>CGIFAYLNYHVPRTRREILETLIKGLQRLEYRGYDSAGVGFDGGNDKDWEANACKIQLIKKKGKVKALDEEVHKQQDMDLDIEFDVHLGIAHTRWATHGEPSPVNSHPQRSDKNNEFIVIHNGIITNYKDLKKFLESKGYDFESETDTETIAKLVKYMYDNRESQDTSFTTLVERVIQQLEGAFALVFKSVHFPGQAVGTRRGDPLLIGVRSEHKLSTDHIPILYRTGKDKKGSCNLSRVDSTTCLFPVEEKAVEYYFASDASAVIEHTNRVIFLEDDDVAAVVDGRLSIHRIKRTAGHHHHHHDHPGRAVQTLQMELQQIMKGNFSSFMQKEIFEQPESVVNTMRGRVNFDDYTVNLGGLKDHIKEIQRCRRLILIACGTSYHAGVATRQVLEELTELPVMVELASDFLDRNTPVFRDDVCFFLSQSGETADTLMGLRYCKERGALTVGITNTVGSSISRETDCGVHINAGPEIGVASTKAYTSQFVSLVMFALMMCDDRISMQERRKEIMLGLKRLPDLIKEVLSMDDEIQKLATELYHQKSVLIMGRGYHYATCLEGALKIKEITYMHSEGILAGELKHGPLALVDKLMPVIMIIMRDHTYAKCQNALQQVVARQGRPVVICDKEDTETIKNTKRTIKVPHSVDCLQGILS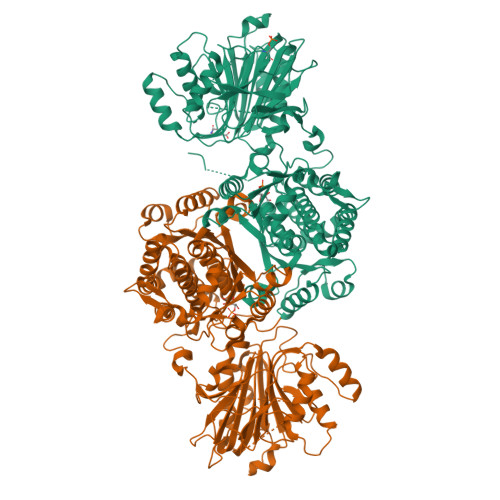VIPLQLLAFHLAVLRGYDVDFPRNLAKSVTVE[2x]> VSPPVLDMDGEPLKIDEEYSIISIPFGGGSVYLANLGNTKCPNGVVQDSSGGNNNKTPVLFYT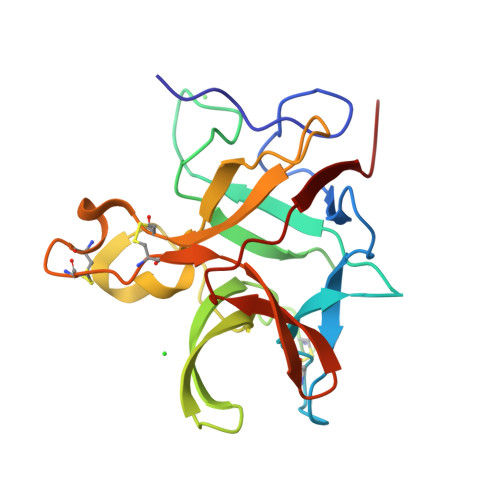MKLGSHFVSENQDVSIKFSTSSSSKSCINETVWKVAYSIVGPTHSPLRFVITGGTFGFPGPNNIENWFKIEKYETGRPHSYKLRYCPSQYICPTCQFDCADVGLYENKGYARLALNNKPYPFGFSKVNKN>VQVNVSFPASVQLHTAVEMHHWCIPFSVDGQPAPSLRWLFNGSVLNETSFIFTEFLEPAANETVRHGCLRLNQPTHVNNGNYTLLAANPFGQASASIMAAFMDNPFE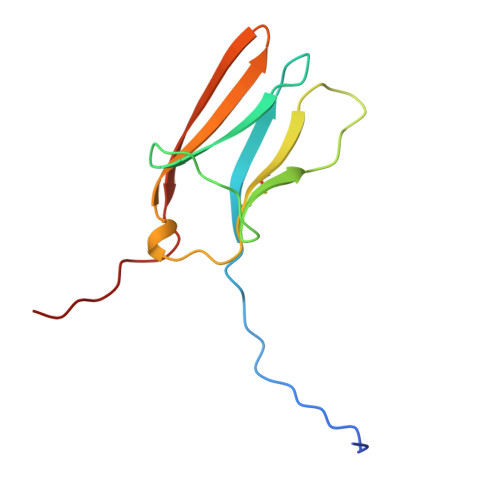FN[2x]>[4x]GSHMELTPDQQTLLHFIMDSYNKQRMPQEITNKILKEAFSAEENFLILTEMAT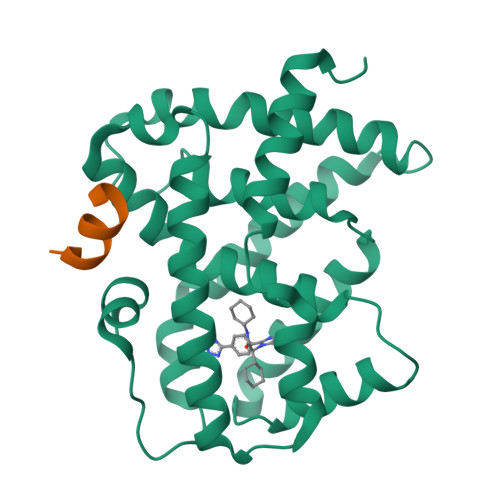NHVQVLVEFTKKLPGFQTLDHEDQIALLKGSAVEAMFLRSAEIFNKKLPSGHSDLLEARIRNSGISDEYITPMFSFYKSIGELKMTQEEYALLTAIVILSPDRQYIKDREAVEKLQEPLLDVLQKLCKIHQPENPQHFACLLGRLTELRTFNHHHAEMLMSWRVNDHKFTPLLCEIWDVQ;>KDHQLLRYLLDKDE[4x]(4R)-3-(4-[4-(2-chlorophenyl)piperazin-1-yl]-6-{[2-methyl-6-(methylcarbamoyl)phenyl]amino}-1,3,5-triazin-2-yl)-N-[2-(hydroxyamino)-2-oxoethyl]-1,3-thiazolidine-4-carboxamide | 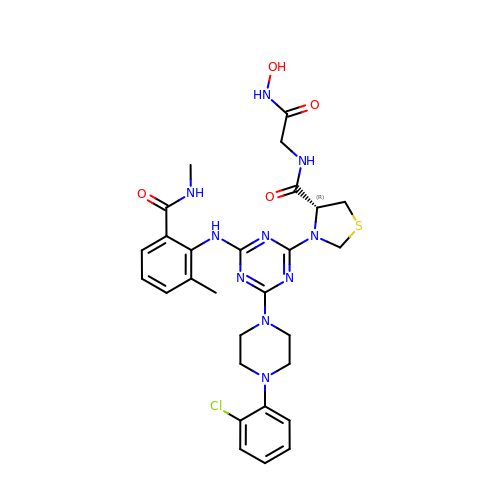C28 H33 Cl N10 O4 S | VJGKWQWGYXBKEJ-NRFANRHFSA-N> AGGGG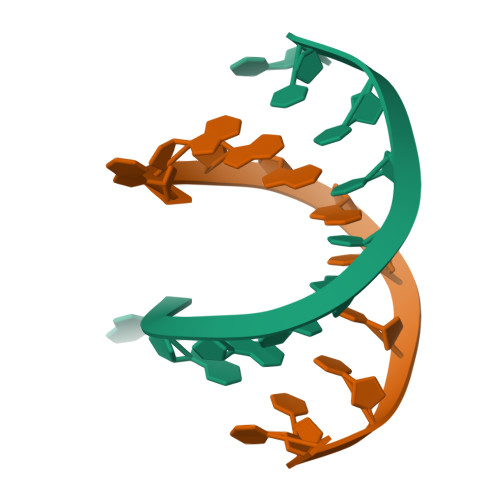CCCCT>TSSANEDMPVERILEAELAVEPKTETYVEANMGLNPSSPNDPVTNICQAADKQLFTLVEWAKRIPHFSELPLDDQVILLRAGWNELLIASFSHRSIAVKDGILLATGLHVHRNSAHSAGVGAIFDRVLTELVSKMRDMQMDKTELGCLRAIVLFNPDSKGLSNPAEVEALREKVYASLEAYCKHKYPEQPGRFAKLLLRLPALRSIGLKCLEHLFFFKLIGDTPIDTFLMEMLEAPHQMT[2x];>TNMGLEAIIRKALMGK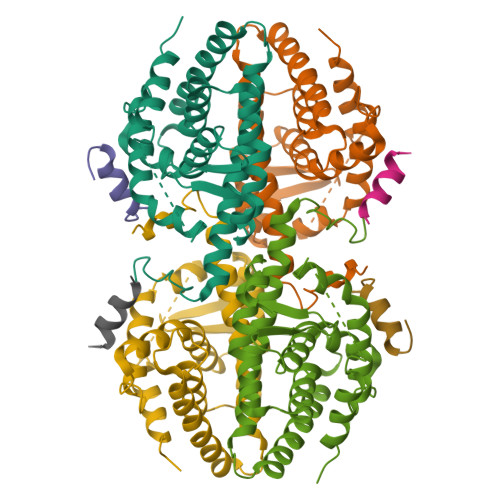[2x]>MLIAIEGVDGAGKRTLVEKLSGAFRAAGRSVATLAFPRYGQSVAADIAAEALHGEHGDLASSVYAMATLFALDRAGAVHTIQGLCRGYDVVILDRYVASNAAYSAARLHENAAGKAAAWVQRIEFARLGLPKPDWQVLLAVSAELAGERSRGRAQRDPGRARDNYERDAELQQRTGAVYAELAAQ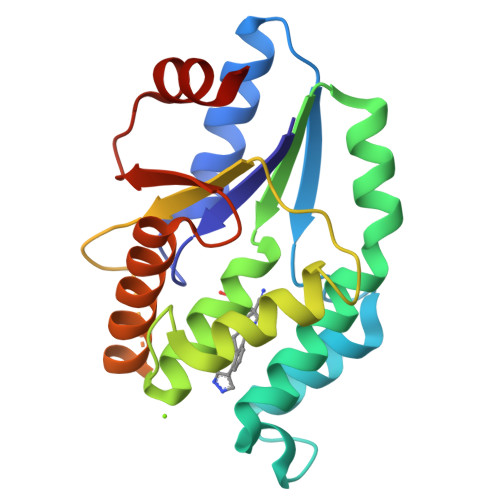GWGGRWLVVGADVDPGRLAATLAPP[2x]>SGSMTSSNRITSPAMTASKTAAVAKPTRAGRKAPAVETAPEASELKMGELSELLGYALKRAQLRVFEDFLHCVAPVQLTPAQFSVLLLLDANPGRNQTEIATTLGILRPNFVAMLDALEGRGLCVRTR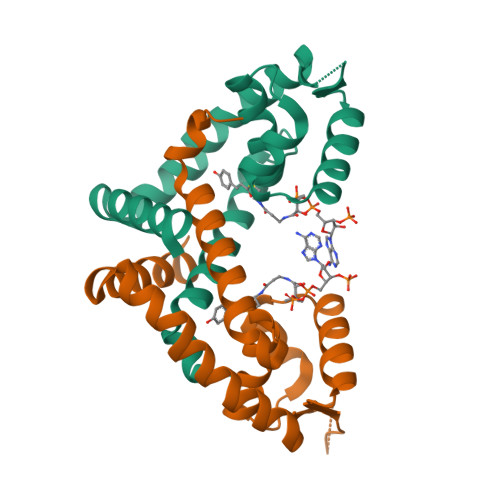SPSDRRSHILMLTDKGRATLARAKKLVATRHEDRLTELLGRDNRDALLSMLATIAREF[4x]> QQEATEVRPEQKMPTLLRVYIDGPHGMGKTTTTQLLVALGSRDDIVYVPEPMTYWRVLGASETIANIYTTQHRLDQGEISAGDAAVVMTSAQITMGMPYAVTDAVLAPHIGGEAGSSHAPPPALTLIFDRHPIAALLCYPAARYLMGSMTPQAVLAFVALIPPTLPGTNIVLGALPEDRHIDRLAKRQRPGERLDLAMLAAIRRVYGLLANTVRYLQCGGSWREDWGQLSGTAVPPQGAE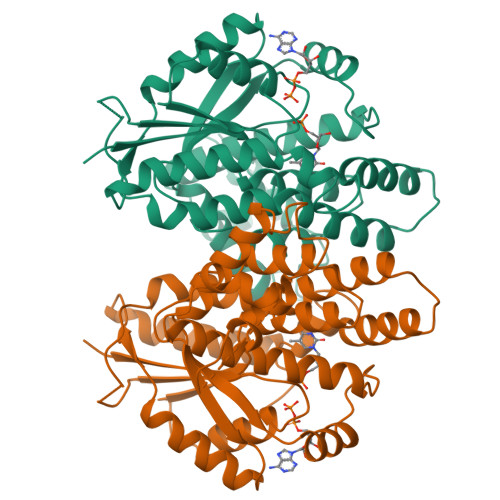PQSNAGPRPHIGDTLFTLFRAPELLAPNGDLYNVFAWALDVLAKRLRSMHVFILDYDQSPAGCRDALLQLTSGMVQTHVTTPGSIPTICDLARTFAREMGEAN>MRFVMPGDRIGSAEEYVKGEGVYEEGGELFAAVAGKLIIKDRVAKVESISPIPEIVKGDVVLGRVVDLRNSIALIEVSSKKGENRGPSNRGIGILHVSNVDEGYVKEISEAVGYLDILKARVIGDNLRLSTKEEEMGVLRALCSNCKTEMVREGDILKCPECGRVEKRKISTDYGKGEW[3x];>MSEFNEKPEKLIVDGLRLDGRKFDELRPIKIEASVLKRADGSCYLEMGKNKVIAAVFGPREVHPEHLQDPSKAIIRYRYNMAPFSVEERKRPGPDRRSIEISKVSKEAFEAVIMKELFPRSAIDIFVEVLQADAGSRTACLNAASVALVDAGVPMKGMITSVAVGKADGQLVLDPMKEEDNFGEADMPFAFLIRNGKIESIALLQMDGRMTRDEVKQAIELAKKGALQIYEMQREAILRRYIEVGEEMDEITEGGEDA[3x];>MPEDILVDIKRDYVLSKLRDNERIDGRGFDEFRKVEIIPNVIEKAEGSALVKLGDTQVVVGVKMQPGEPAPDTPDRGVIIVNAELVPLASPTFEPGPPDENSIELARVVDRGIRESEAVDLSKLVIEEGEKV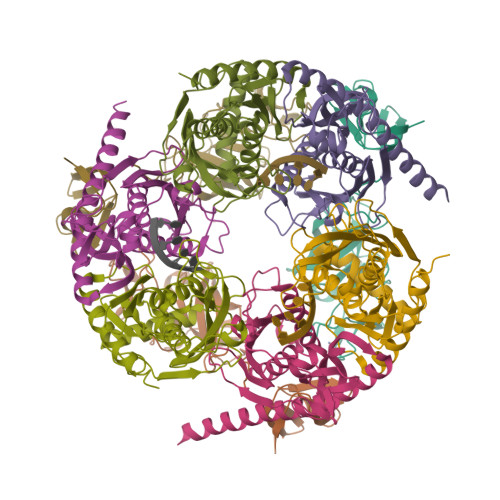WIVFVDIHALDDDGNLLDASALAAIAALMNTKVPAERFDLGEDYLLPVRDLPVSVTSLIVGNKYLVDPSREEMSVGDTTLTITTDKDDNVVAMQKSGGYLLDEKLFDELLDVSINCARKLREKFKEI[3x]>MSTLIEAIVAREVLDSRGNPTIEVDVRLESGDVGRAIVPSGASTGAHEALELRDGDKSRYNGKGVLKAVQAVNEDIAEALIGFDAADQIALDQELIALDGTPNKSKLGANAILGVSLAAAKAAAAAFGLPLYRYLGGVYAHVLPVPMMNIMNGGQHATNSTDFQEFMIMPVGAESFREGLRWGAEIYHMLKKVIHDRGFSTTVGDEGGFAPSLPTNDAPLQLIMEAIEKAGYRPGEQIVIALDPATTEIFEDGKYHLKREGRSLSSAEMVDYWVDLVN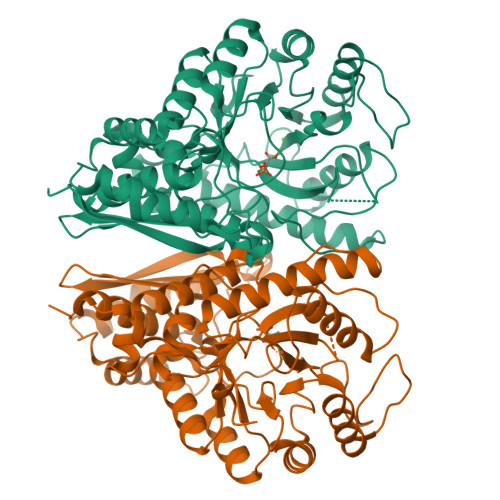RYPIISLEDGLAEDDWEGWALLRAKLGDRVQLVGDDFLVTNVQRLQRAIEAKAANSILIKLNQIGSLTETLSAIQLAQRSGWTAVVSHRSGESEDVTIADLVVATNAGQIKTGAPARTDRIAKYNQLLRIEEELGSAARYAGRSAFKV[2x]>GSHMASMTGGQQMGRGSNEEFRPEMLQGKKVIVTGASK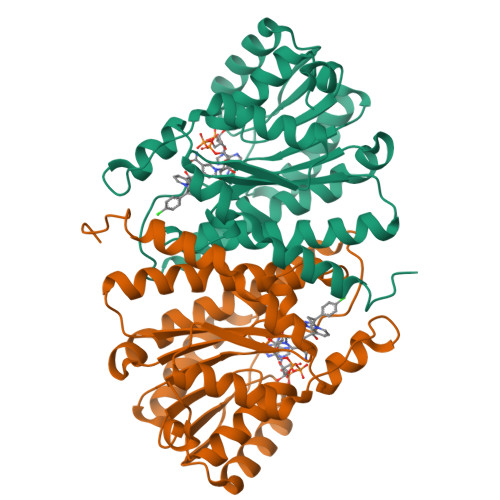GIGREMAYHLAKMGAHVVVTARSKETLQKVVSHCLELGAASAHYIAGTMEDMTFAEQFVAQAGKLMGGLDMLILNHITNTSLNLFHDDIHHVRKSMEVNFLSYVVLTVAALPMLKQSNGSIVVVSSLAGKVAYPMVAAYSASKFALDGFFSSIRKEYSVSRVNVSITLCVLGLIDTETAMKAVSGIVHMQAAPKEECALEIIKGGALRQEEVYYDSSRWTTLLIRNPCRKILEELYSTSYNMDRFINK[4x]> SMLRPRLCTMKKGPSGYGFNLHSDKSKPGQFIRS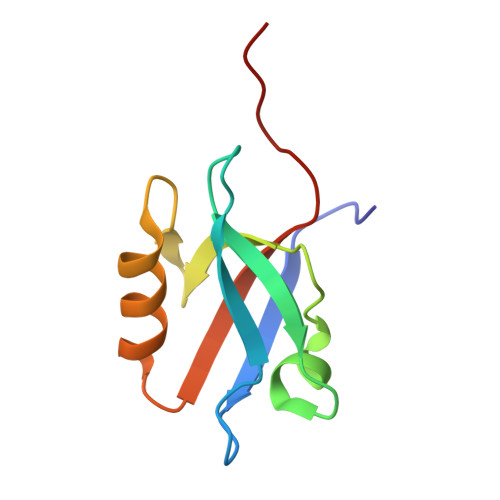VDPDSPAEASGLRAQDRIVEVNGVCMEGKQHGDVVSAIRAGGDETKLLVVDRETETSL>[2x]MLESKLKAPVFTATTQGDHYGEFVLEPLERGFGVTLGNPLRRILLSSIPGTAVTSVYIEDVLHEFSTIPGVKEDVVEIILNLKELVVRFLDPKMASTTLILRAEGPKEVRAVDFTPSADVEIMNPDLHIATLEEGGKLYMEVRVDRGVGYVPAERHGIKDRINAIPVDAIFSPVRRVAFQVEDTRLGQRTDLDKLTLRIWTDGSVTPLEALNQAVAILKEHLNYFANPEASSLPTPEVSKGEKRESAEEDLDLPLEELGLSTRVLHSLKEEGIESVRALLALNLKDLRNIPGIGERSLEEIRQALAKKGFTLKE;> MKIKRFGRIREVIPLPPLTEIQVESYKKALQADVPPEKRENVGIQAAFKETFPIEEGDKGKGGLVLDFLEYRIGDPPFSQDECREKDLTYQAPLYARLQLIHKDTGLIKEDEVFLGHLPLMTEDGSFIINGADRVIVSQIHRSPGVYFTPDPARPGRYIASIIPLPKRGPWIDLEVEASGVVTMKVNKRKFPLVLLLRVLGYDQETLVRELSAYGDLVQGLLDEAVLAMRPEEAMVRLFTLLRPGDPPKKDKALAYLFGLLADPKRYDLGEAGRYKAEEKLGVGLSGRTLVRFEDGEFKDEVFLPTLRYLFALTAGVPGHEVDDIDHLGNRRIRTVGELMADQFRVGLARLARGVRERMVMGSPDTLTPAKLVNSRPLEAALREFFSRSQLSQFKDETNPLSSLRHKRRISALGPGGLTRERAGFDVRDVHRTHYGRICPVETPEGANIGLITSLAAYARVDALGFIRTPYRRVKNGVVTEEVVYMTASEEDRYTIAQANTPLEGDRIATDRVVARRRGEPVIVAPEEVEFMDVSPKQVFSLNTNLIPFLEHDDANRALMGSNMQTQAVPLIRAQAPVVMTGLEERVVRDSLAALYAEEDGEVVKVDGTRIAVRYEDGRLVHPLRRYARSNQGTAFDQRPRVRVGQRVKKGDLLADGPASEEGFLALGQNVLVAIMPFDGYNFEDAIVISEELLKRDFYTSIHIERYEIEARDTKLGPERITRDIPHLSEAALRDLDEEGIVRIGAEVKPGDILVGRTSFKGEQEPSPEERLLRSIFGEKARDVKDTSLRVPPGEGGIVVGRLRLRRGDPGVELKPGVREVVRVFVAQKRKLQVGDKLANRHGNKGVVAKILPVEDMPHLPDGTPVDVILNPLGVPSRMNLGQILETHLGLAGYFLGQRYISPVFDGATEPEIKELLAEAFNLYFGKRQGEGFGVDKREKEVLARAEKLGL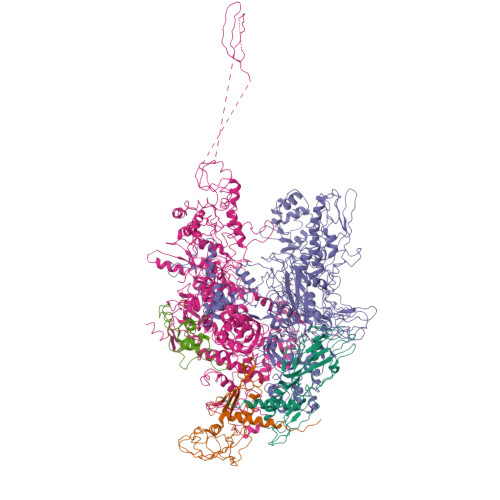VSPGKSPEEQLKELFDLGKVVLYDGRTGEPFEGPIVVGQMFIMKLYHMVEDKMHARSTGPYSLITQQPLGGKAQFGGQRFGEMEVWALEAYGAAHTLQEMLTIKSDDIEGRNAAYQAIIKGEDVPEPSVPESFRVLVKELQALALDVQTLDEKDNPVDVFEGLASKR;> MKKEVRKVRIALASPEKIRSWSYGEVEKPETINYRTLKPERDGLFDERIFGPIKDYECACGKYKRQRFEAKVCERCAVEVTRSIVRRYRMAHIELATPAAHIWFVKDVPSKIATLLDLSATELEQVLYFNKYIVLDPKAAVLDAVPVEKRQLLTDXXXXXXXXXXXXXXXXXXXXXXXXXXXXXXXXXXXXIDARMGAEAIQELLKELDLEKLERELLEEMKHPSRARRAKARKRLEVVRAFLDSGNRPEWMILEAVPVLPPDLRPMVQVDGGRFATSDLNDLYRRLINRNNRLKKLLAQGAPEIIIRNEKRMLQEAVDAVIDNGRRGSPVTNPGSERPLRSLTDILSGKQGRFRQNLLGKRVDYSGRSVIVVGPQLKLHQCGLPKRMALELFKPFLLKKMEEKAFAPNVKAARRMLERQRDIKDEVWDALEEVIHGKVVLLNRAPTLHRLGIQAFQPVLVEGQSIQLHPLVCEAFNADFDGDQMAVHVPLSSFAQAEARIQMLSAHNLLSPASGEPLAKPSRDIILGLYYITQVRKEKKGAGMAFATPEEALAAYERGEVALNAPIVVAGRETSVGRLKFVFANPDEALLAVAHGLLDLQDTVTTRYLGRRLETSPGRILFARIVGEAVGDEKVAQELIQMDVPQEKNSLKDLVYQAFLRLGMEKTARLLDALKYYGFTLSTTSGITIGIDDAVIPEEKQRYLEEADRKLRQIEQAYEMGFLTDRERYDQVIQLWTETTEKVTQAVFNNFEENYPFNPLYVMAQSGARGNPQQIRQLCGMRGLMQKPSGETFEVPVRSSFREGLTVLEYFISSHGARKGGADTALRTADSGYLTRKLVDVAHEIVVREADCGTTNYISVPLFQMDEVTRTLRLRKRSDIESGLYGRVLAREVEALGRRLEEGRYLSLEDVHFLIKAAEAGEVREVPVRSPLTCQTRYGVCQKCYGYDLSMARPVSIGEAVGVVAAESIGEPGTQLTMRTFHTGGVAVGTDITQGLPRVIELFEARRPKAKAVISEIDGVVRIEEGEDRLSVFVESEGFSKEYKLPKDARLLVKDGDYVEAGQPLTRGAIDPHQLLEAKGPEAVERYLVDEIQKVYRAQGVKLHDKHIEIVVRQMLKYVEVTDPGDSRLLEGQVLEKWDVEALNERLIAEGKVPVAWKPLLMGVTKSALSTKSWLSAASFQNTTHVLTEAAIAGKKDELIGLKENVILGRLIPAGTGSDFVRFTQVVDQRTLKAIEEARKEAVEAKEKEAPRRPVRREQPGKGL;> MAEPGIDKLFGMVDSKYRLTVVVAKRAQQLLRHRFKNTVLEPEERPKMRTLEGLYDDPNAVTWAMKELLTGRLFFGENLVPEDRLQKEMERLYPTEEEA>[4x]GSMPLLLDDGDPKAQTGFDLST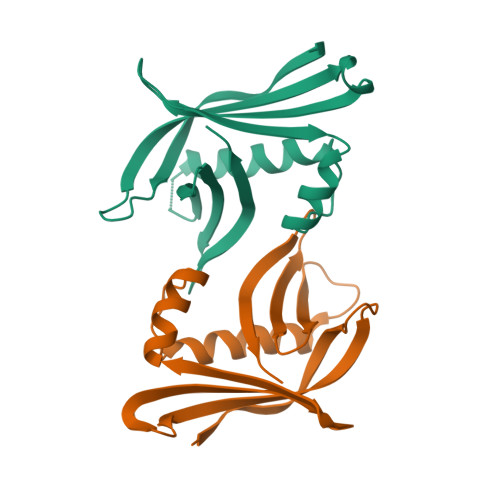ATTLFWRPVPVHVKQQDREDVLEELTFRILTGVAKQNHNLRILRIHISSDSDLFFLHTLEVSEEDFQSLKNDQEILVDFASFPGKIISLLEKCILAQPGDSPRFQAVLTIRGGESVFKIVEINDWKKLPHITLAFRPGN> MGSDAFDEMDEIWALYADDGAQALDAMEASLLALQAGEDAAAHVGPLFRAVHTFKGNSRVLGLSVVESRAHLCEDLIGLVRDAGVPMDGEIVEILLFASDTLRAMLEETAASRADVEGTGSEALMDQLRSKIARCSRSHHHHHH;> MRGSHHHHHHGSPYNVMIVDDAAMMRLYIASFIKTLPDFKVVAQAANGQEALDKLAAQPNVDLILLDIEMPVMDGMEFLRHAKLKTRAKICMLSSVAVSGSPHAARARELGADGVVAKPSGTVSHDLEEKTGGELARTMRTLMAA

Two-component pathways comprise sensor histidine kinases (HPK) and response regulators (RRs). Once phosphorylated, the HPK transfers the phosphoryl group to an aspartate residue within the receiver domain of the cognate RR. Neither CheA3 nor CheA4 is capable of autophosphorylation; instead, CheA4 phosphorylates CheA3 on H51 of the P1 (Hpt) domain. Once phosphorylated, CheA3-P serves as a specific phosphodonor for the chemotaxis RRs, CheY1, CheY6, and CheB2.

In order to elucidate the molecular details of the interaction between CheA3 and CheY6, the complex structure of CheY6 and the unphosphorylated Hpt domain of CheA3 (residues 1–135) has been solved to 1.40 Å using Seleno single-wavelength anomalous dispersion (SAD) for phasing. CheY6 has the typical (α/β)5 topology seen for E. coli CheY and other structurally characterized RRs. Although crystallized in the presence of Mn2+, there was no additional density in the CheY6 divalent cation binding site. CheA3P1 forms a four-helix bundle (αA–αD) with an additional C-terminal helix (αE). The site of phosphorylation, His51 in CheA3P1, is located on αB, in close proximity to the active site of the RR with the phosphoacceptor Asp56 on CheY6 being 7.5Å from His51 on CheA3P1. The interface between CheA3P1 and CheY6 is dominated by hydrophobic interactions with only one hydrogen bond and no salt bridges formed between the two proteins. The buried surface area of the interface is small (530 Å2), indicative of a weak interaction, consistent with the transient nature of the complexes. In this region, helices αA and αB of CheA3P1 form a hydrophobic pocket comprising Ile11, Leu14, and Tyr15 on αA, and Asn56, Val59, and Leu60 on αB. This pocket is situated adjacent to α1 on CheY6 and in ideal position to accommodate Met13 on the N-terminal region of this helix.>MGLFAGKGVLVTGGARGIGRAIAQAFAREGAL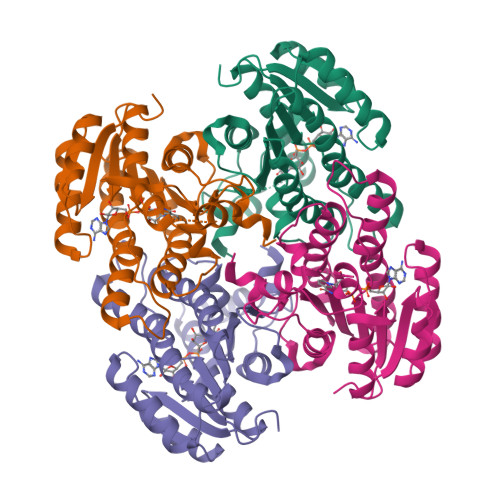VALCDLRPEGKEVAEAIGGAFFQVDLEDERERVRFVEEAAYALGRVDVLVNNAAIAAPGSALTVRLPEWRRVLEVNLTAPMHLSALAAREMRKVGGGAIVNVASVQGLFAEQENAAYNASKGGLVNLTRSLALDLAPLRIRVNAVAPGAIATEAVLEAIALSPDPERTRRDWEDLHALRRLGKPEEVAEAVLFLASEKASFITGAILPVDGGMTASFMMAGRPV[4x]>[2x]GAASKKVNVLVVGLDNSGKTTIIERLKPRPRQAAEVAPTVGFTVDEVEKGPLTFTVFDMSGAGRYRTLWEQ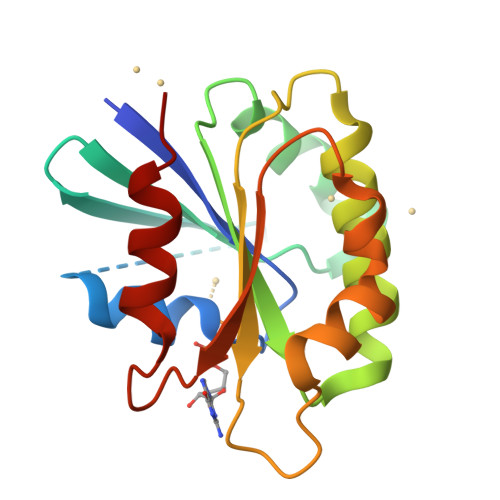YYREADAVVFVVDSADKLRMVVARDEMEHMLKHSNMRKVPILYFANKKDLPVAMPPVEIAQALGLDDIKDRPWQIVPSNGLTGEGVDKGIDWLAERLS>[2x]MLVLVIGDFHVPHRSAAIPQVFLDRLNTGRIQTVLCTGNLCGKETYDILRTLAREVHVVKGDFDEMQGLNETEVIKIGNFKIGLMHGHQVIPWGDREALAIYQRQ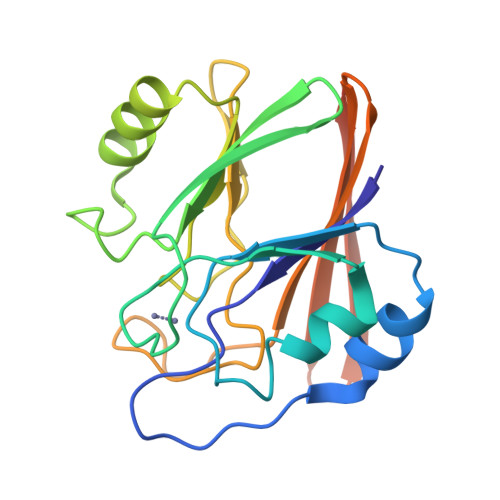LDVDILITGHTHKLETKEVGGKYFLNPGSATGAYSPLVDNPVPSFMLLEINDSELTIYEYTLVDGSVKCERVDFNKKQQQLEHHHHHH> MRGSHHHHHHGMAEPLLVVGLGNPGANYARTRHNLGFVVADLLAARLGAKFKAHKRSGAEVATGRSAGRSLVLAKPRCYMNESGRQIGPLAKFYSVAPANIIVIHDDLDLEFGRIRLKIGGGEGGHNGLRSVVAALGTKDFQRVRIGIGRPPGRKDPAAFVLENFTPAERAEVPTICEQ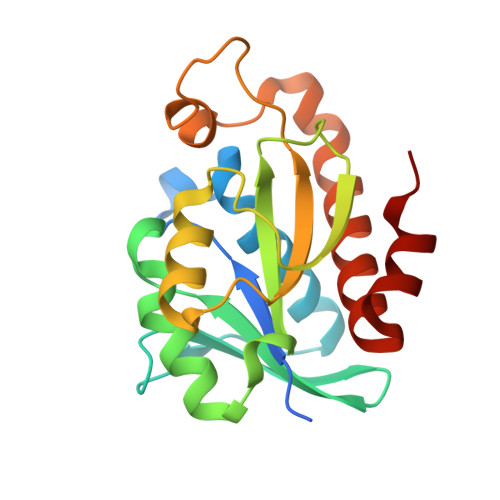AADATELLIEQGMEPAQNRVHAW> LALQAKQYGDFDRYVLALSWQTGFCQSQHDRNRNERDECRL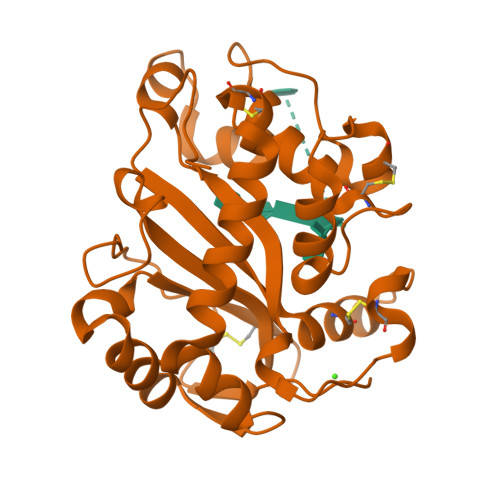QTETTNKADFLTVHGLWPGLPKSVAARGVDERRWMRFGCATRPIPNLPEARASRMCSSPETGLSLETAAKLSEVMPGAGGRSCLERYEYAKHGACFGFDPDAYFGTMVRLNQEIKESEAGKFLADNYGKTVSRRDFDAAFAKSWGKENVKAVKLTCQGNPAYLTEIQISIKADAINAPLSANSFLPQPHPGNCGKTFVIDKAGY> MLNKSFVKKLDESLNRKQVGSTNVTRYKIEDSYLVLAAVRVGIGGLTYHNGAAHFLEHLKFWRYGENIYNLFFQRGAILNAYTTLEFTDYVFLSKEESINENLNLLLTFLYHHQYDEKTISLERNIIINEINGAGTARLNGQESIEKERHCILGSAESISRMGRKEFELI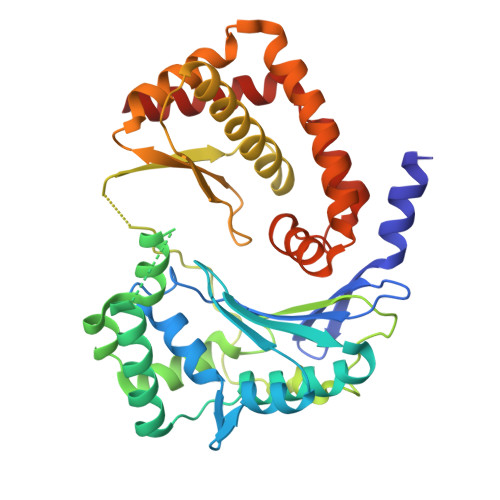SQKYYTPENTSIYVIGGNQDIDLFHIPTAVMTTQYGKPTHKVNVNEVEMNKDMILLPVEHGDYLKNRMICHLIADMIKHLAQQLEYDVSVGLFISTNQHSCYLKVKKSDQKRFSSLIQQLSMDEHFIETYIKDYQWRFMNELVINFNQLHNIYDYMTEYRLGEYTVAELFGSLDSVDKLDILAVRNELINQLTVGE> MSELLDSFETEFAKFYTDSNLEETNLQKCLDHTHEFKSQLKKLKAHLNKHIQESKPEVYNKLSDKEKQKFKRKRELIIEKLSKSQRQWDHSVKKQIKYVSQQSNRFNKSTLNKLKEFDIDSVYVNKLPKETMENVNEAIGYHILRYSIDNMPLGNKNEAFQYLKDVYGITNKESTEFIEMGQIVHDLKKGDTESCLKWCS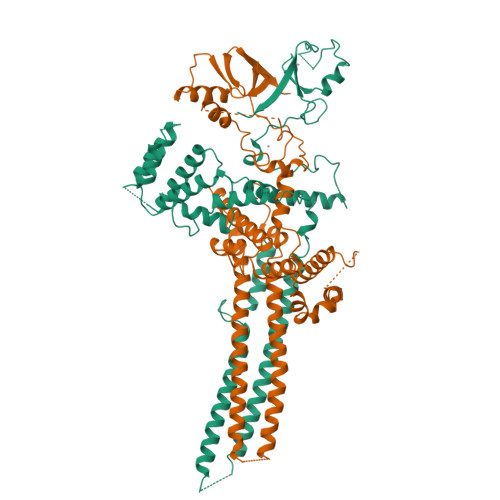NEMESLSSNHTALSSLKFDLYTLSAMQIVKHGNPVELYYQITQNAPLDCFRHREKELMQNVVPLLTKSLIGQPIEDIDSKVNKELKECTSLFIKEYCAAKHIFFDSPLFLIVLSGLISFQFFIKYKTIRELAHVDWTTKDELPFDVKLPDFLTHFHPIFICPVLKEETTTENPPYSLACHHIISKKALDRLSKNGTITFKCPYCPVNTSMSSTKKVRFVML;> MAEKSIFNEPDVDFHLKLNQQLFHIPYELLSKRIKHTQAVINKETKSLHEHTAALNQIFEHNDVEHDELALAKITEMIRKVDHIERFLNTQIKSYCQILNRIKKRLEFFHELKDIKSQNSGTSHNGNNEGTRTKLIQWYQSYTNILIGDYLTRNNPIKYNSETKDHWNSGVVFLKQSQLDDLIDYDVLLEANRISTSLLHERNLLPLISWINENKKTLTKKSSILEFQARLQEYIELLKVDNYTDAIVCFQRFLLPFVKSNFTDLKLASGLLIFIKYCNDQKPTSSTSSGFDTEEIKSQSLPMKKDRIFQHFFHKSLPRITSKPAVNTTDYDKSSLINLQSGDFERYLNLLDDQRWSVLNDLFLSDFYSMYGISQNDPLLIYLSLGISSLKTRDCLHPSDDENGNQETETATTAEKEVEDLQLFTLHSLKRKNCPVCSETFKPITQALPFAHHIQSQLFENPILLPNGNVYDSKKLKKLAKTLKKQNLISLNPGQIMDPVDMKIFCESDSIKMYPT> TKGLVLGIYSKEKEEDEPQFTSAGENFNKLVSGKLREILNISGPPLKAGKTRTFYGLHEDFPSVVVVGLGKKTAGIDEQENWHEGKENIRAAVAAGCRQIQDLEIPSVEVDPCGDAQAAAEGAVLGLYEYDDLKQKRKVVVSAKLHGSEDQEAWQRGVLFASGQNLARRLMETPANEMTPTKFAEIVEENLKSASIKTDVFIRPKSWIEEQEMGSFLSVAKGSEEPPVFLEIHYKGSPNASEPPLVFVGKGITFDSGGISIKAAANMDLMRADMGGAATICSAIVSA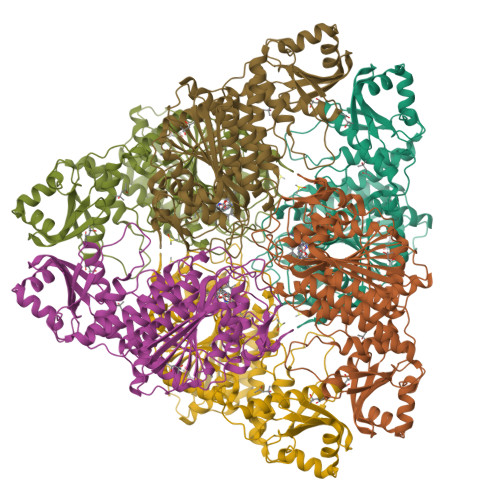AKLDLPINIVGLAPLCENMPSGKANKPGDVVRARNGKTIQVDNTDAEGRLILADALCYAHTFNPKVIINAATLTGAMDIALGSGATGVFTNSSWLWNKLFEASIETGDRVWRMPLFEHYTRQVIDCQLADVNNIGKYRSAGACTAAAFLKEFVTHPKWAHLDIAGVMTNKDEVPYLRKGMAGRPTRTLIEFLFRFSQESA;> ALYY>[2x]GALIEHHAASSTDQPVDVPYNLDMFSQAAVLAQETYCGEQAHDYGLKLGDATLLWTAGDGNVRQRVNLYQSDSLGIAVAIQGTNTSSLRSDLHDAQLRPVDPDSRYRRFLPQGTKVMNGFQKGYTDLVDDIFDHVKKFKQEKNESRVTVIGHSLGAAIGLLASLDINL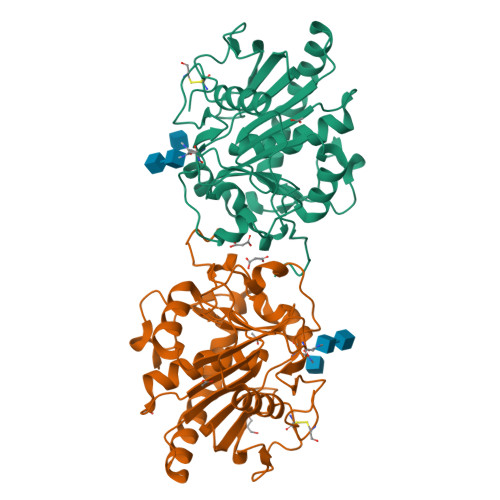RLEDGLFKSYLFGLPRVGNPIFANFVDRKIGDKLHWVVNGRDWVPTVPPRALGYQHPSNYVWIYPANSTNWKLYPGQENVHGMLTVAREFNFDDHEGIYFHTQIGASLGKCPAVLGGY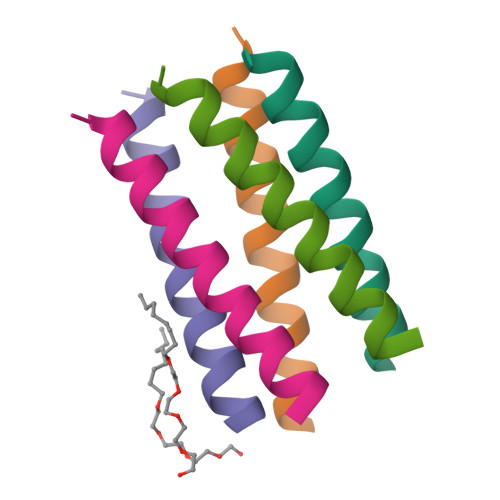>[15x]DSQKWIVFLLFLIVLLLLAIVFLLRG>[3x]HMFEARLVQGSILKKVLEALKDLINEACWDISSSGVNLQSMDSSHVSLVQLTLRSEGFDTYRCDRNLAMGVNLTSMSKILKCAGNEDIITLRAEDNADTLALVFEAPNQEKVSDYEMKLMDLDVEQLGIPEQEYSCVVKMPSGEFARICRDLSHIGDAVVISCAKDGVKFSASGELGNGNIKLSQTSNVDKEEEAVTIEMNEPVQLTFALRYLNFFTKA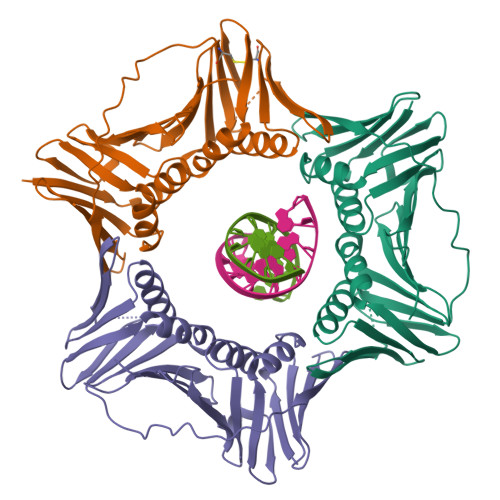TPLSSTVTLSMSADVPLVVEYKIADMGHLKYYLAPKIEDEEGS> FTPINSSQWIANGNASIFPDKLLLTTDDYGEAGSVWYYKPVNLSEDLVVEFYAYLGDNPDGADGITFTLQSLGTNEL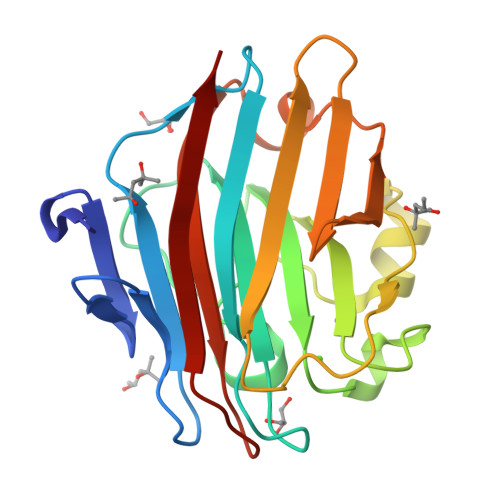GGTGGDLGYGGISPSVAVEVDTWLNDFDAPATTDHIAIDVNGNINHTYNSLTYPTPNPYDLGNVEDGREHLIKIVWNATTKTLQVYFDGNLSLTWNKDITQIIGNSAYFGFTGGTGGAKNLQYVKPIYVKNG>[2x]MSPEI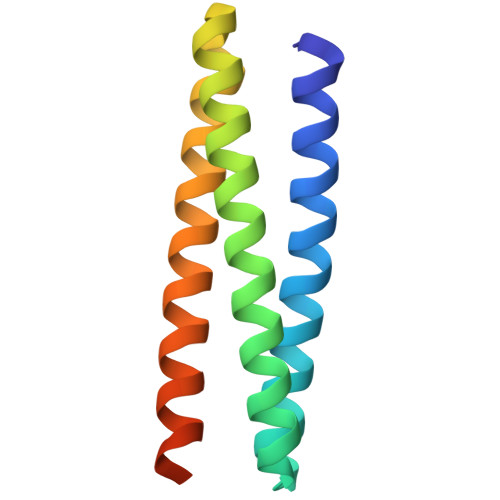EDLLKKILELLEKAFALWAEAKKALAEGDLEKAISTLKELIATIEEVIVLTKKALELAEKEGNPEIVEQAKKLLDLAEALLEAAKAELARALSLNPLEHHHHHH> XTVFTSWEEYLD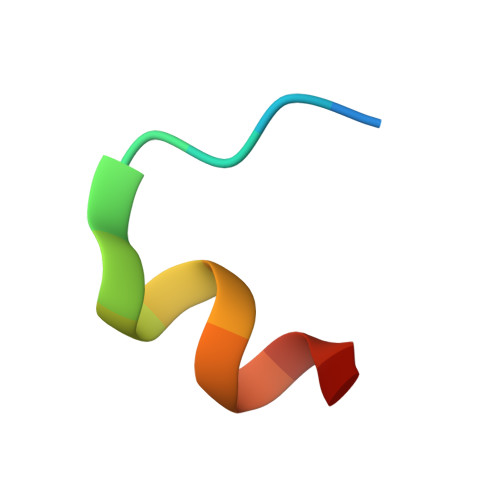WVX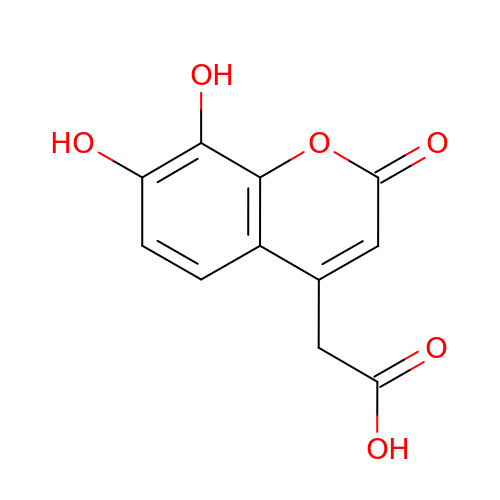(7,8-dihydroxy-2-oxo-2H-chromen-4-yl)acetic acid | C11 H8 O6 | LNRFNPKOQGRTFS-UHFFFAOYSA-N> DPDTAVTNKQSFSTDVIYQVFTDRFLDGNPSNNPTGAAYDATCSNLKLYCGGDWQGLINKINDNYFSDLGVTALWISQPVENIFATINYSGVTNTAYHGYWARDFKKTNPYFGTMADFQNLITTAHAKGIKIVIDFAPNHTSPADAENGRLYDNGTLVGGYTNDTNGYFHHNGGSDFSSLENGIYKNLYDLADFNHNNATIDKYFKDAIKLWLDMGVDGIRVDAVKHMPLGWQKSWMSSIYAHKPVFTFGEWFLGSAASDADNTDFANKSGMSLLDFRFNSAVRNVFRDNTSNMYALDSMINSTATDYNQVNDQVTFIDNHDMDRFKTSAVNNRRLEQALAFTLTSRGVPAIYYGTEQYLTGNGDPDNRAKMPSFSKSTTAFNVISKLAPLRKSNPAIAYGSTQQRWINNDVYVYERKFGKSVAVVAVNRNLSTSASITGLSTSLPTGSYTDVLGGVLNGNNITSTNGSINNFTLAAGATAVWQYTTAETTPTIGHVGPVMGKPGNVVTIDGRGFGSTKGTVYFGTTAVTGAAITSWEDTQIKVTIPSVAAGNYAVKVAASGVNSNAYNNFTILTGDQVTVRFVVNN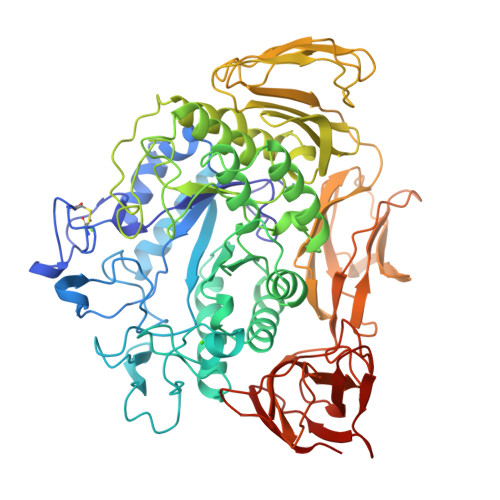ASTTLGQNLYLTGNVAELGNWSTGSTAIGPAFNQVIHQYPTWYYDVSVPAGKQLEFKFFKKNGSTITWESGSNHTFTTPASGTATVTVNWQ> MKKLLALGLLGLVLASCGKKEETTTGPKETTIFAMHLGKALDPNLPVFVKAEKDTNIKLVNVASQNQTDQIQAYNLMLTEGKLPDIVSYELSADLENLGIEGGLIPLEDLINQHAPNLKKFFEENPRYKKDAVAVDGHIYMIPNYYDYFNIKVS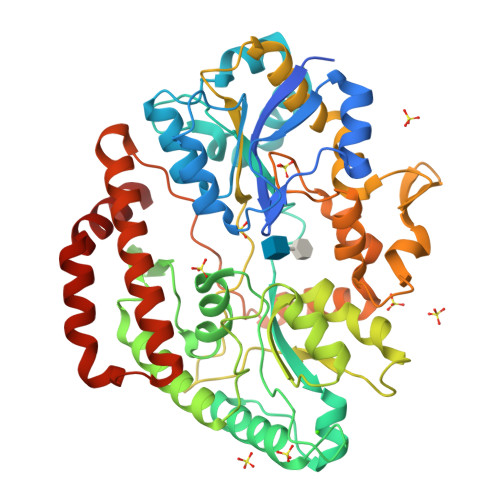QGYFIRQDWLEKLGLKEPRTVDELYTTLKAFREKDPNGNGKKDEVPFFVRANNVRKVLTSLVDLFKASPIWYEENGMVKYGPAQKEFKHAIKELSKWYKEGLIDEEIFTRGLESRDYLLSNNLGGATDDWIASTSSYNRNLADKIPGFNLKLVLPYELNGNAKTRHARTTYLGGWGISKDAKDPVSLIKYFDYWYSVEGRRLWNFGIEGSEYTLVDGKPVFTDKVLKNPDGKTPLAVLREVGAQYRLGAFQDAQYELGWASESAKAGYKYYMDNDVVLDELPILKYTKEKSKEFVSIDTAMRAVVEEKAQQWILGSGDIDKEWDAYIKRLENLGLSKAEQIQNEAFKNFNK> MTQAKAKHADVPVNLYRPNAPFIGKVISNEPLVKEGGIGIVQHIKFDLTGGNLKYIEGQSIGIIPPGVDKNGKPEKLRLY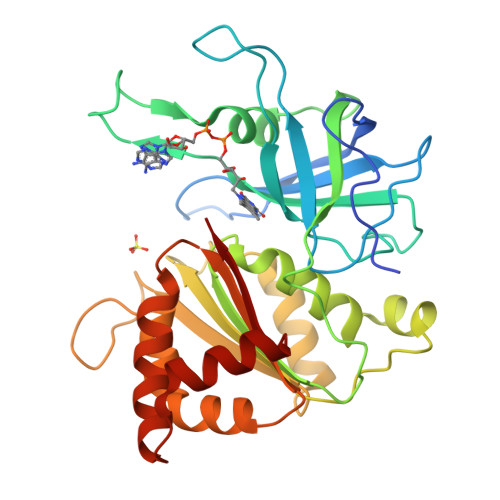SIASTRHGDDVDDKTISLCVRQLEYKHPESGETVYGVCSTYLTHIEPGSEVKITGPVGKEMLLPDDPEANVIMLAGGTGITPMRTYLWRMFKDAERAANPEYQFKGFSWLVFGVPTTPNILYKEELEEIQQKYPDNFRLTYAISREQKNPQGGRMYIQDRVAEHADQLWQLIKNQKTHTYICGPRGMEEGIDAALSAAAAKEGVTWSDYQKDLKKAGRWHVETY> MRYRKGARDTAFLVLYRWDLRGENPGELFKEVVEEKNIKNKDAYEYAKKLVDTAVRHIE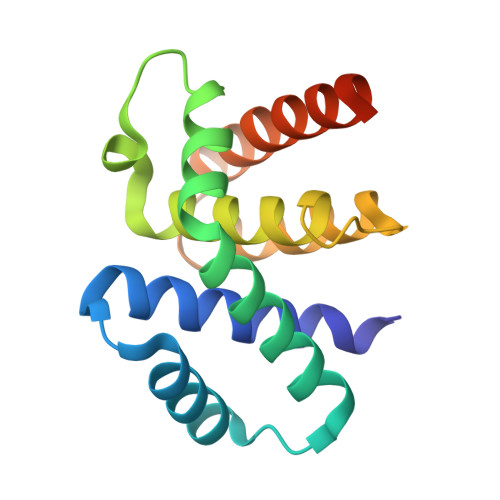EIDSIIEKHLKGWSIDRLGYVERNALRLGVAELIFLKSKEPGRVFIDIVDLVKKYADEKAGKFVNGVLSAIYKAYITSSKEEKPSLKSE>GSMAVTNVAELNALVERVKKAQREYASFTQEQVDKIFRAAALAAADARIPLAKMAVAESGMGIVEDKVIKNHFASEYIYNAYKDEKTCGVLSEDDTFGTITIAEPIGIICGIVPTTNPTSTAIFKSLISLKTRNAIIFSPHPRAKDATNKAADIVLQAAIAAGAPKDLIGWIDQPSVELSNALMHHPDINLILATGGPGMVKAAYSSGKPAIGVGAGNTPVVIDETADIKRAVASVLMSKTFDNGVICASEQSVVVVDSVYDAVRERFATHGGYLLQGKELKAVQDVILKNGALNAAIVGQPAYKIAELAGFSVPENTKILIGEVTVVDESEPFAHEKLSPTLAMYRAKDFEDAVEKAEKLVAMGGIGHTSCLYTDQDNQPARVSYFGQKMKTARILINTPASQGGIGDLYNFKLAPSLTLGCGSWGGNSISENVGPKHLINKKTVAKRAENMLWHKLPKSIYFRRGSLPIALDEVITDGHKRALIVTDRFLFNNGYADQITSVLKAAGVETEVFFEVEADPTLSIVRKGAELANSFKPDVIIALGGGSPMDAAKIMWVMYEHPETHFEELALRFMDIRKRIYKFPKMGVKAKMIAVTTTSGTGSEVTPFAVVTDDATGQK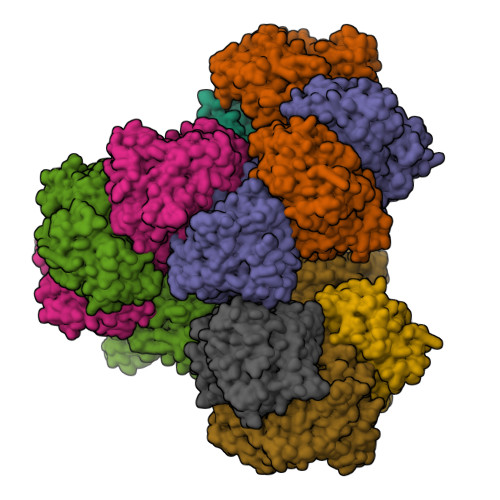YPLADYALTPDMAIVDANLVMDMPKSLCAFGGLDAVTHAMEAYVSVLASEFSDGQALQALKLLKEYLPASYHEGSKNPVARERVHSAATIAGIAFANAFLGVCHSMAHKLGSQFHIPHGLANALLICNVIRYNANDNPTKQTAFSQYDRPQARRRYAEIADHLGLSAPGDRTAAKIEKLLAWLETLKAELGIPKSIREAGVQEADFLANVDKLSEDAFDDQCTGANPRYPLISELKQILLDTYYGRDYVEGETAAKKEAAPAKAEKKAKKSA[8x]Here, we show that repeat number variation in predicted bacterial surface proteins is more widespread and we characterize a third rod-like repetitive region in the Streptococcus gordonii protein (Sgo_0707) formed by tandem array of Streptococcal High Identity Repeats in Tandem (SHIRT) domains. The structure of single and tandem SHIRT domains from the streptococcal surface protein Sgo_0707 were determined. We call SasG, Rib, and Sgo_0707 “Periscope Proteins” due to their having variable-length stalk-like regions that define the distance that the N-terminal functional domain projects from the bacterial surface. Taken together, these data are consistent with multiple tandemly arrayed SHIRT domains from Sgo_0707 behaving as an elongated, rod-like particle.

Based on the significant truncation of the N-terminal β-strand (Inset), we hypothesized that shifting the frame of the repeat by seven residues toward the N terminus of Sgo_0707 would complete the fold. Sgo_R3 (residues 621 through 705) and Sgo_R10 (residues 1211 through 1299) based on this new definition were thus expressed and purified. The model confirms that SHIRT has an α/β fold organized around a single α-helix and two distinct β-sheets. We report the 3D structure of a SHIRT domain which, while also containing β-sheets, has a topology with no obvious relationship to the Ig fold.

>[2x]VTHKAVHEFVSGTPGKELPQEVKALLPVDQTDLKDGIQVTPTQPSQTEVKTSEGTWSFKSYDKTSETVNGSDVKFVGTWEFTASPAPT> GPLSLSVDAFKILEDPKWEFPRKNLVLGKTLGEGEFGKVVKATAFHLKGRAGYTTVAVKMLKENASPSELRDLLSEFNVLKQVNHPHVIKLYGACSQDGPLLLIVEYAKYGSLRGFLRESRKVGPGYLGSGGSRNSSSLDHPDERALTM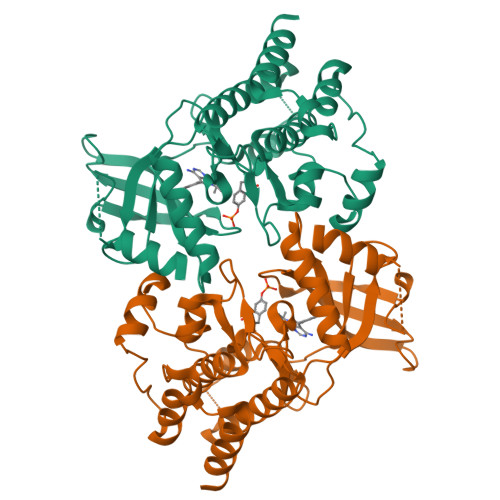GDLISFAWQISQGMQYLAEMSLVHRDLAARNILVAEGRKMKISDFGLSRDVYEEDSYVKRSQGRIPVKWMAIESLFDHIYTTQSDVWSFGVLLWEIVTLGGNPYPGIPPERLFNLLKTGHRMERPDNCSEEMYRLMLQCWKQEPDKRPVFADISKDLEKMMVKRR> MGRFIFVSFGLLVVFLSLSGTGADVDCLPGWSAYDQSCYRVFKLLKTWDDAE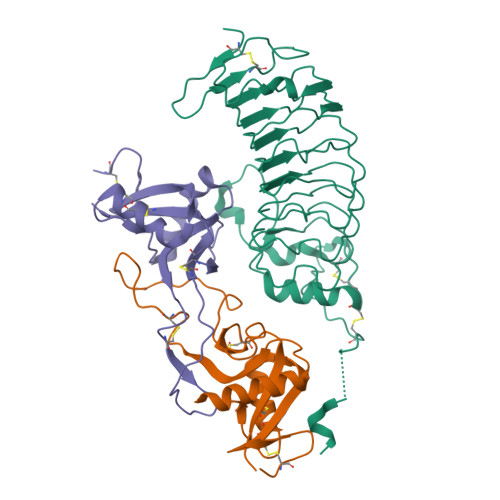KFCTERPKGGHLVSIESAGERDFVAQLVSENKQTDNVWLGLKIQSKGQQCSTEWTDGSSVSYENFSEYQSKKCFVLEKNTGFRTWLNLNCGSEYAFVCKSPP;> MGRFIFVSFGLLVVFLSLRGTGAGFCCPLRWSSYEGHCYLVVKEKKTWDDAEKFCTEQRKGGHLVSVHSREEADFLVHLAYPILDLSLIWMGLSNMWNDCKREWSDGTKLDFKAWAKTSDCLIGKTDGDNQWLNMDCSKKHYFVCKFKL;> HPICEVSKVASHLEVNCDKRQLTALPPDLPKDTTILHLSENLLYTFSLATLMPYTRLTQLNLDRCELTKLQVDGTLPVLGTLDLSHNQLQSLPLLGQTLPALTVLDVSFNRLTSLPLGALRGLGELQELYLKGNELKTLPPGLLTPTPKLEKLSLANNQLTELPAGLLNGLENLDTLLLQENSLYTIPKGFFGSHLLPFAFLHGNPWLCNCEILYFRRWLQDNAENVYVWKQGVDVKAMTSNVASVQCDNSDKFPVYKYPGKGCPTLGDEGDTDLYDYYPEEDTEGDKVRATRTVVKFPTKAHTT>MDHKVHHHHHHIEGRHMDSLITFEKLTAQHLPY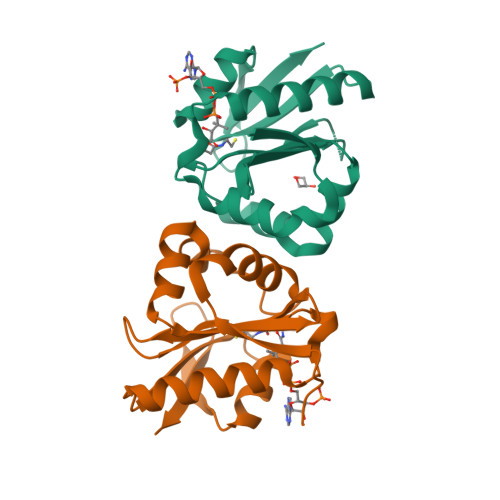LYEIRFSVEENLLHPHQIQYLQRRQALEDINQGGGWICKHGDDYAGVGFGLFIPEPLIGGLFVKPEYQSKGIGSALLARVTAWMFERGAEAIHLTTDPGSKAEGFYQHHGWAVVGQDEFGQAELVKRKEGE[2x]> MADLNWETVISSDSSPAVENEHPQETPESNNSVYTSFMKSHRCYDLIPTSSKLVVFDTSLQVKKAFFALVTNGVRAAPLWD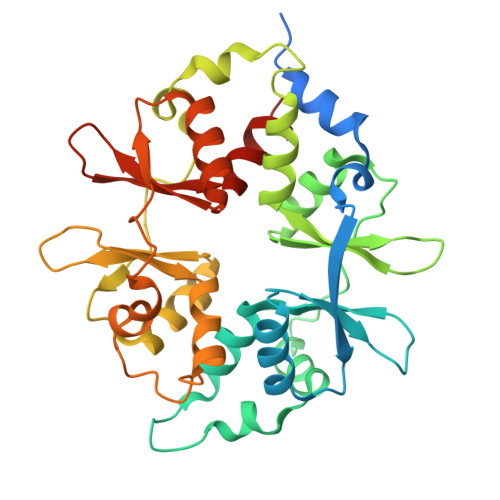SKKQSFVGMLTITDFINILHRYYKSALVQIYELEEHKIETWREVYLQDSFKPLVCISPNASLFDAVSSLIRNKIHRLPVIDPESGNTLYILTHKRILKFLKLFITEFPKPEFMSKSLEELQIGTYANIAMVRTTTPVYVALGIFVQHRVSALPVVDEKGRVVDIYSKFDVINLAAEKTYNNLDVSVTKALQHRSHYFEGVLKCYLHETLETIINRLVEAEVHRLVVVDENDVVKGIVSLSDILQALVLTGGEKKP>[2x]MGSSHHHHHHSSGLVPRGSHMERPQLDSMSQDLSEALKEATKEVHIRAENSEFMRNFQKGQVSREGFKLVMASLYHIYTALEEEIERNKQNPVYAPLYFPEELHRRAALEQDMAFWYGPHWQEAIPYTPATQHYVKRLHEV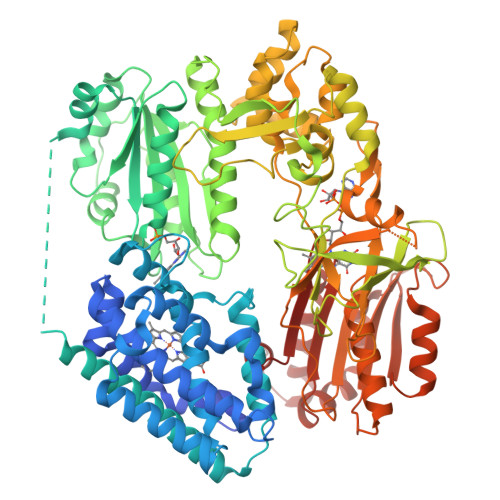GGTHPELLVAHAYTRYLGDLSGGQVLKKIAQKAMALPSSGEGLAFFTFPSIDNPTKFKQLYRARMNTLEMTPEVKHRVTEEAKTAFLLNIELFEELQALLPEEHKDQSASQTEFLRMQTTAPPVKESSFVEKMKKTGRNIIVFYGSQTGTAEEFANRLSKDAHRYGMRGMSADPEEYDLADLSSLPEIDKSLVVFCMATYGEGDPTDNAQDFYDWLQETDVDLTGVKFAVFGLGNKTYEHFNAMGKYVDQRLEQLGAQRIFELGLGDDDGNLEEDFITWREQFWPAVCEFFGVEASSIRQYELVVHEDMDVAKVYTGEMGRLKSYENQKPPFDAKNPFLAAVTANRKLNQGTERHLMHLELDISDSKIRYESGDHVAVYPANDSALVNQIGEILGADLDVIMSLNNLDEESNKKHPFPCPTTYRTALTYYLDITNPPRTNVLYELAQYASEPSEQEHLHKMASSSGEGKELYLSWVVEARRHILAILQDYPSLRPPIDHLCELLPRLQARYYSIASSSKVHPNSVHICAVAVEYEAKSGRVNKGVATSWLRAKEPAGENGGRALVPMFVRKSQFRLPFKSTTPVIMVGPGTGIAPFMGFIQERAWLREQGKEVGETLLYYGCRRSDEDYLYREELARFHKDGALTQLNVAFSREQAHKVYVQHLLKRDREHLWKLIHEGGAHIYVCGDARNMAKDVQNTFYDIVAEFGPMEHTQAVDYVKKLMTKGRYSLDVWS>GPGSRIAEEAVGNVSTGALRTITLSKMKQSLGISISGGIESKVQPMVKIEKIFPGGAAFLCGDLQAGFELVAVDGESLEQVTHQRAVDTIRRAYRNKAREPMELVVRVP[2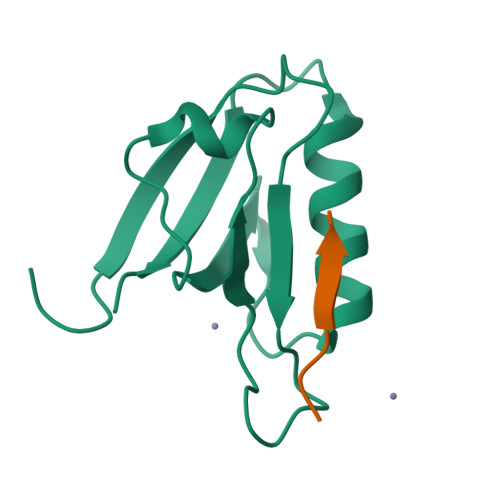x];>[2x]GPGSTEKMEDVEITLV acetylene | C2 H2 | 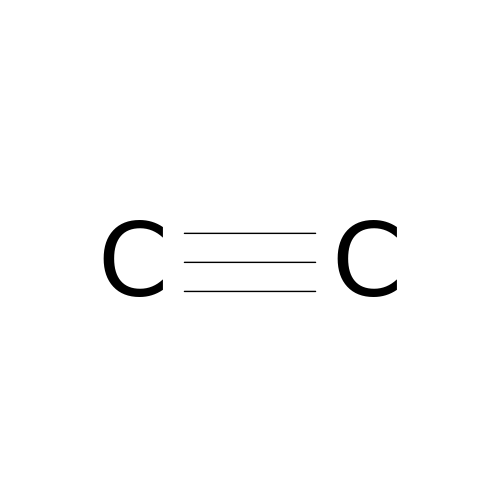HSFWRNGVRCDJHI-UHFFFAOYSA-N>MVSC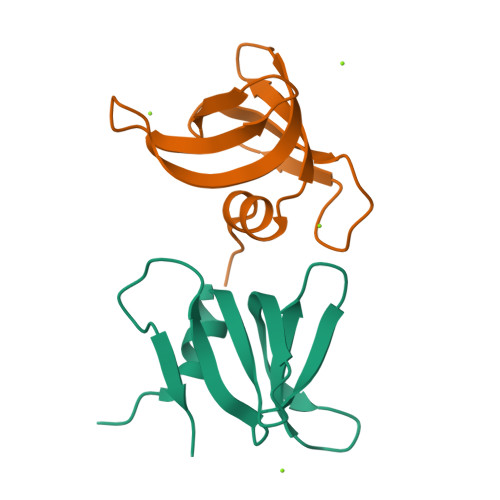SQYDYIELACLFHLPVKLTMKSGEVYYGVAADTQRNSQKQECIALRGEEETWLLETDQLSSMEALSEQPHFSVIHFK[2x]~{N}-(4-chlorophenyl)-4-methyl-piperidine-1-carboxamide | 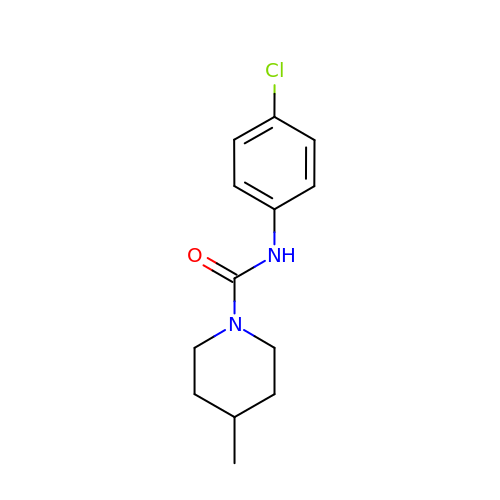C13 H17 Cl N2 O | WMWBLCFXKIUSDK-UHFFFAOYSA-N>KMAKDSKAPVVEIFDERDGCTSAGSTGKASDAGEKGLLVKVSMQKVGYNAIMAKSVAASYMNK[2x];>[2x]MLDAFSKVITSADGKAAYVGGADLQALKKFVSDGNKRMDAVNAIVSNASCIVSDAVSGMVCENPSLIAPNGGVYSNRKMAACLRDAEIILRYVSYSLLSGDSSVLEDRCLNGLKETYSSLGVPAAGNARAVAIMKATVNSFINNTAQQKKLSVPSGDCSALASEAGGYFDKVTSAIG

In addition to their membrane‐bound chlorophyll a/c light‐harvesting antenna, the cryptophyte algae have evolved a unique phycobiliprotein antenna system located in the thylakoid lumen. The basic unit of this antenna consists of two copies of an αβ protomer where the α and β subunits scaffold different combinations of a limited number of linear tetrapyrrole chromophores. While the β subunit is highly conserved, encoded by a single plastid gene, the nuclear‐encoded α subunits have evolved diversified multigene families. By careful examination of three newly determined crystal structures in comparison with three previously obtained, we show how the α subunit amino acid sequences control chromophore conformations and hence spectral properties even when the chromophores are identical.

The crystal structure of PC577 from H. pacifica CCMP706 has been determined at 1.0 Å resolution. The structure shows a two‐fold symmetric (αβ)2 complex that adopts the open form quaternary structure which is closest to that of PC612 from H. virescens (RMSD 0.531 Å over 2909 atoms; cf., PE555 from H. andersenii—RMSD 0.670 Å over 2657 atoms). The atomic resolution electron density map shows unequivocally that PC577 has the same chromophores as PC612. The chromophore structures are also near identical with only a slight twist between pyrrole ring C and ring D in the β158 PCB which is quantified by a difference in dihedral angles linking the rings: (−13 ± 6°, +12 ± 1°). The loop protecting the α20 PCB chromophore from the solvent is different in the two structures and it is marked by a distinct sequence in each protein (residues 21–27 following Cys20, which is the covalent chromophore attachment site). In PC577, this segment forms a single helical turn, making multiple hydrogen bonds to the α20 chromophore. Thus, the α20 PCB in PC577 is highly constrained by the protein. The backbone carbonyl group of Gly24 in PC577 forms a hydrogen bond to the nitrogen atom of pyrrole ring D in the α20 chromophore. This results in a −10° rotation of the inner dihedral angle linking ring C to ring D in PC577 when compared to PC612. Thus, the differences in amino acid sequence between the α subunits of PC577 and PC612 are likely to be responsible for the observed spectral differences.> AMHPRKDWYELTRATNWTPSYVTEEQLFPERMSGHMGIPLEKWESYDEPYKTSYPEYVSIQREKDAGAYSVKAALERAKIYENSDPGWISTLKSHYGAIAVLEYAAVTGEGRMARFSKAPGNRNMATFGMMDELRHGQLQLFFPHEYCKKDRQFDWAWRAYHSNEWAAIAAKHFFDDIITGRDAISVAIMLTFSFETGFTNMQFLGLAADAAEAGDYTFANLISSIQTDESRHAQQGGPALQLLIENGKREEAQKKVDMAIWRAWRLFAVLTGPVMDYYTPLEDRSQSFKEFMYEWIIGQFERSLIDLGLDKPWYWDLFLKDIDELHHSYHMGVWYWRTTAWWNPAAGVTPEERDWLEEKYPGWNKRWGRCWDVITENVLNDRMDLVSPETLPSVCNMSQIPLVGVPGDDWNIEVFSLEHNGRLYHFGSEVDRWVFQQDPVQYQNHMNIVDRFLAGQIQPMTLEGALKYMGFQSIEEMGKDAHDFAWADKCK;> SFESKKPMRTWSHLAEMRKKPSEYDIVSRKLHYSTNNPDSPWELSPDSPMNLWYKQYRNASPLKHDNWDAFTDPDQLVYRTYNLMQDGQESYVQSLFDQFNEREHDQMVREGWEHTMARCYSPLRYLFHCLQMSSAYVQQMAPASTISNCCILQTADSLRWLTHTAYRTHELSLTYPDAGLGEHERELWEKEPGWQGLRELMEKQLTAFDWGEAFVSLNLVVKPMIVESIFKPLQQQAWENNDTLLPLLIDSQLKDAER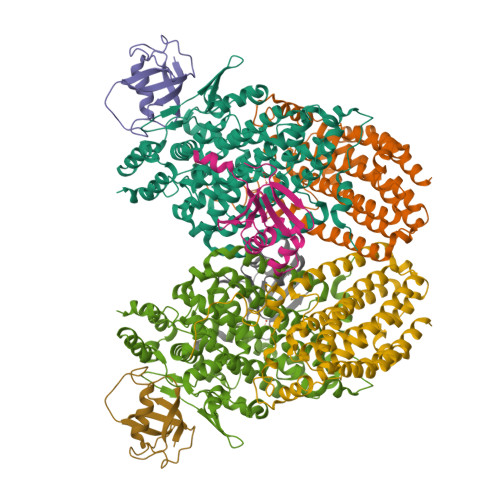HSRWSKALVKHALENPDNHAVIEGWIEKWRPLADRAAEAYLSMLSS;> SAFPVHAAFEKDFLVQLVVVDLNDSMDQVAEKVAYHCVNRRVAPREGVMRVRKHRSTELFPRDMTIAESGLNPTEVIDVVFEE;> TLADQALHNNNVGPIIRAGDLVEPVIETAEIDNPGKEITVEDRRAYVRIAAEGELILTRKTLEEQLGRPFNMQELEINLASFAGQIQADEDQIRFYFDKTM> MAHHHHHHMTQSVCILGVTGSIGRSTLKILGQHPD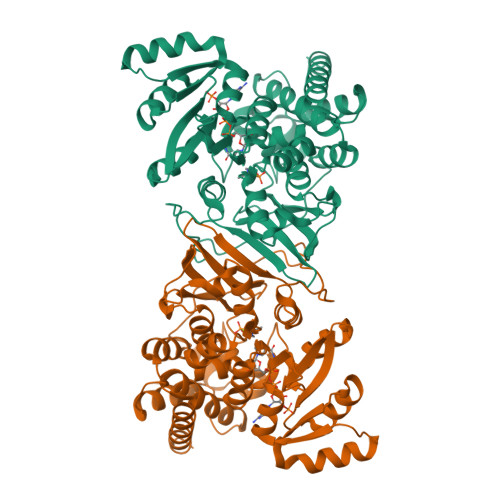KYSVFAVSAHSRISELVEICKQFRPKVVVVPEQKIAELKTLFAQQNISDIDVLAGQEGLVDIASHTDVDIVMAAIVGAAGLLPTLAAVKAGKRVLLANKEALVMSGEIMMQAARDHQALLLPVDSEHNAIFQSLPHNYLQADRTGQPQLGVSKILLTASGGPFLNHSLEQLVHVTPQQACKHPNWSMGQKISVDSATLMNKGLELIEACHLFSISEHFVTVVVHPQSIIHSMVQYVDGSTLAQMGNPDMCTPIAHALAWPERLQTNVPALDLFEYSQLNFQAPDTQKFPALNLARQAMRAGGLAPTILNAANEIAVEAFLMERIGFTSIPQVVEHTLEKLENAAAESIECILDKDKVARSVAQQYISSIGG>[2x]MSSSNVEVFIPVSQGNTNGFPATASNDLKAFTEGAVLSFHNICYRVKLKSGFLPCRKPVEKEILSNINGIMKPGLNAILGPTGGGKSSLLDVLAARKDPSGLSGDVLINGAPRPANFKCNSGYVVQDDVVMGTLTVRENLQFSAALRLATTMTNHEKNERINRVIQELGLDKVADSKVGTQFIRGVSGGERKRTSIGMELITDPSILFLDEPTTGLDSSTANAVLLLLKRMSKQGRTIIFSIHQPRYSIFKLFDSLTLLASGRLMFHGPAQEALGYFESAGYHCEAYNNPADFFLDIINGDSTAVALNREEDFKATEIIEPSKQDKPLIEKLAEIYVNSSFYKETKAELHQLSGGEKKKKITVFKEISYTTSFCHQLRWVSKRSFKNLLGNPQASIA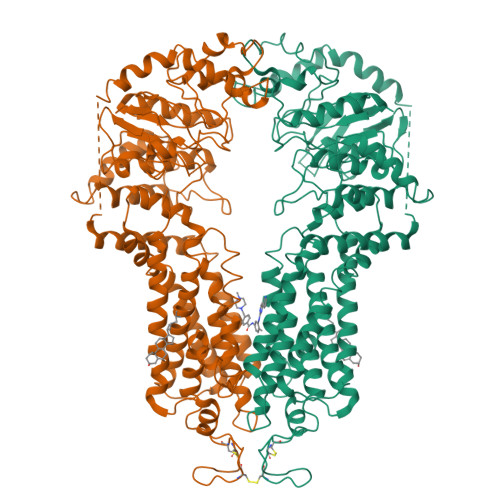QIIVTVVLGLVIGAIYFGLKNDSTGIQNRAGVLFFLTTNQCFSSVSAVELFVVEKKLFIHEYISGYYRVSSYFLGKLLSDLLPMRMLPSIIFTCIVYFMLGLKPKADAFFVMMFTLMMVAYSASSMALAIAAGQSVVSVATLLMTICFVFMMIFSGLLVNLTTIASWLSWLQYFSIPRYGFTALQHNEFLGQNFCPGLNATGNNPCNYATCTGEEYLVKQGIDLSPWGLWKNHVALACMIVIFLTIAYLKLLFLKKYS>[2x]M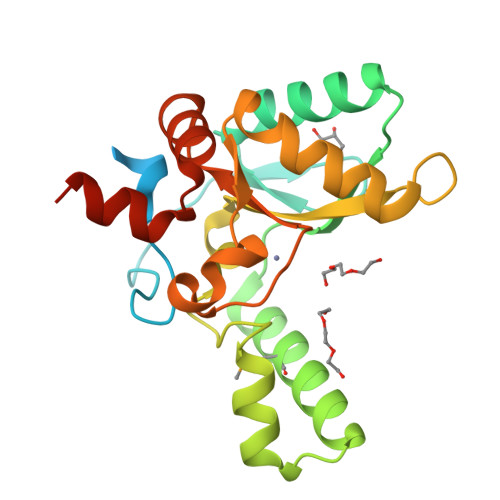ASTQLPPIPATHTGSGTGVAENPEENTLATAKEQGDEQEWSLILVNRQNPIPAQYDVELEQLSNGERIDIRISPYLQDLFDAARADGVYPIVASGYRTTEKQQEIMDEKVAEYKAKGYTSAQAKAEAETWVAVPGTSEHQLGLAVDINADGIHSTGNEVYRWLDENSYRFGFIRRYPPDKTEITGVSNEPWHYRYVGIEAATKIYHQGLCLEEYLNTEKLEHHHHHH> RLNSQRLVFNRPF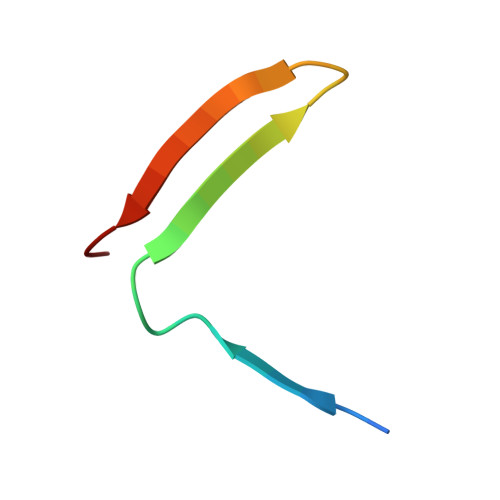LMFIVDNNILFLGKVNRP> ITI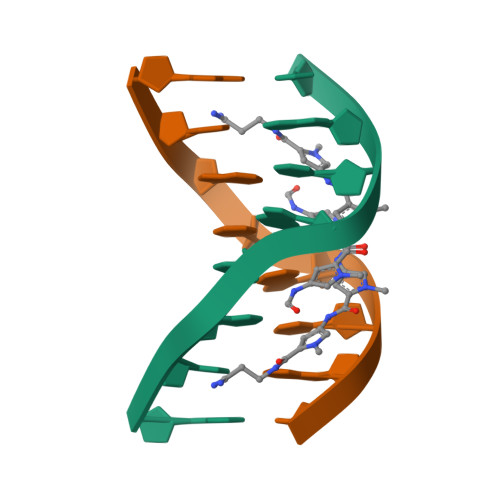TACAC>[2x]MSSSNACASPSPFPAV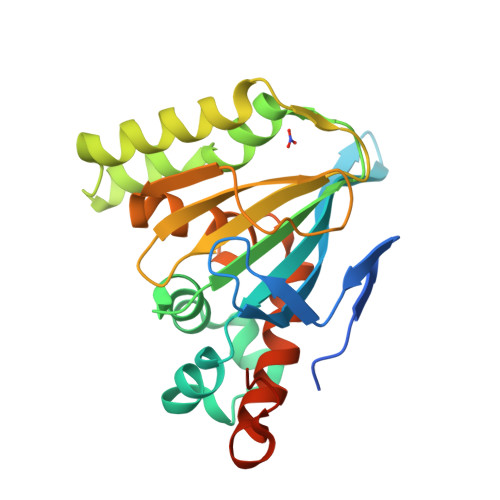TKLHVDSVTFVPSVKSPASSNPLFLGGAGVRGLDIQGKFVIFTVIGVYLEGNAVPSLSVKWKGKTTEELTESIPFFREIVTGAFEKFIKVTMKLPLTGQQYSEKVTENCVAIWKQLGLYTDCEAKAVEKFLEIFKEETFPPGSSILFALSPTGSLTVAFSKDDSIPETGIAVIENKLLAEAVLESIIGKNGVSPGTRLSVAERLSQLMMKNKDEKEVSDHSVEEKLAKEN>[2x]MASNDPGNEVSSYSPTSPSYVKF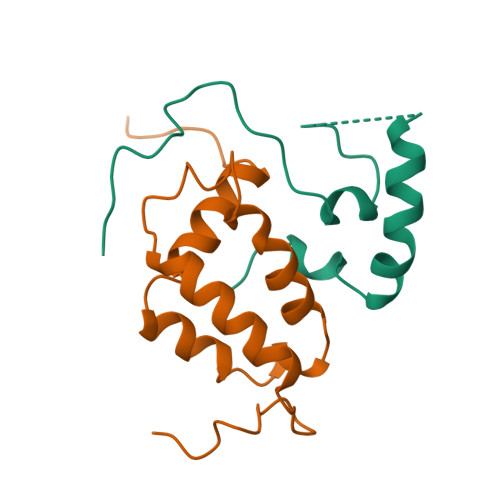FTQSNLEKLPKYKEKKAASAKQTAPNNSNGGSEEEITCALDYLIPPPMPKNQQYRAFGSIW;>[2x]GSHMSSTNGNAPATPSSDQNPLPTRFEVELEFIQSLANIQYVTYLLTQQQIWKSPNFKNYLKYLEYWCNPPYSQCIVYPNCLFILKLLNGFMESAIVNEDGLLEGLDELPKIIQLQGPQWMNEMVERWAN> VPRGSHMTRLDSVERAVADIAAGKAVIVIDDEDRENEGDLIFAAEKATPEMVAFMVRYTSGYLCVPLDGAICDRLGLLPMYAVNQDKHGTAYTVTVDARNG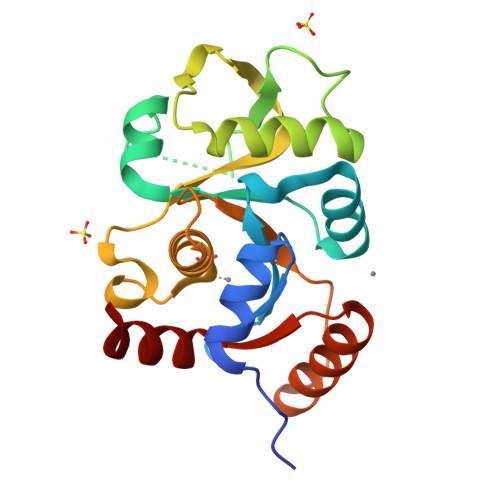IGTGISASDRATTMRLLADPTSVADDFTRPGHVVPLRAKDGGVLRRPGHTEAAVDLARMAGLQPAGAICEIVSQKDEGSMAHTDELRVFADEHGLALITIADLIEWRRKHE>[6x]HHHHHHSSGLVPRGS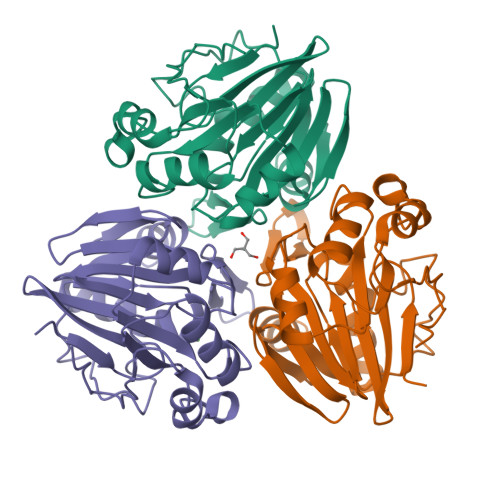HMMKLSFHGQSTIYLEGNNKKVIVDPFISNNPKCDLNIETVQVDYIVLTHGHFDHFGDVVELAKKTGATVIGSAEMADYLSSYHGVENVHGMNIGGKANFDFGSVKFVQAFHSSSFTHENGIPVYLGMPMGIVFEVEGKTIYHTGDTGLFSDMSLIAKRHPVDVCFVPIGDNFTMGIDDASYAINEFIKPKISVPIHYDTFPLIEQDPQQFKDAVNVGDVQILKPGESVQF>CACCTAGCGA[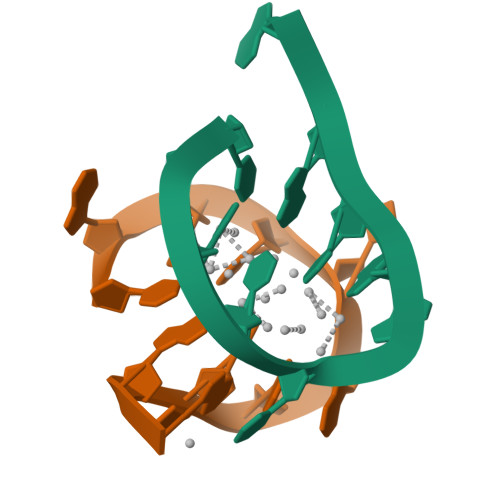4x]>[2x]PDPMKNTCKLLVVADHRFYRYMGRGEESTTTNYLIELIDRVDDIYRNTAWDNAGFKGYGIQIEQIRILKSPQEVKPGEKHYNMAKSYPNEEKDAWDVKMLLEQFSFDIAEEASKVCL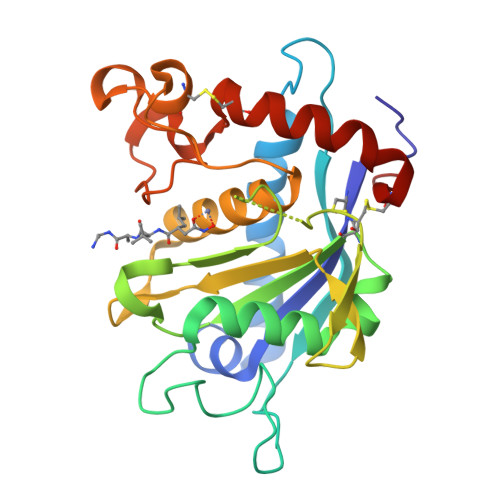AHLFTYQDFDMGTLGLAYGGSPRANSHGGVCPKAYYSPVGKKNIYLNSGLTSTKNYGKTILTKEADLVTTHELGHNFGAEHDPDGLAECAPNEDQGGKYVMYPIAVSGDHENNKMFSQCSKQSIYKTIESKAQECFQERSN>MFKTEFEFPEELKTKLQEHINYFPKKRQAILLCLHEIQNYYGYIPPESLKPLADMLELPLNHVEGVVAFYDMFDREDKAKYRIRVCVSIVCHLMGTNKLLKALENILGIKPGEVTPDGKFKIVPVQCLGACSEAPVFMVNDDEYKFESEVQLNEILSRYT[2x];>MRSYPAIPRIYAETTLNMLLKRAKKPRVHSIDEYLKDGGYQALEKALNMSPEEIIDWVDKSTLRGRGGAGFPTGKKWKFAVQNPGPRYFICNADESEPGTFKDRIIIERDPHLLIEGIIISSYAIGANEAYIYIRGEYPAGYYILRDAIEEAKKKGFLGKNILGSGFDLEIYVARGAGAYICGEETALIESLEGKRGHPRLKPPYPVQKGLWGKPTVVNNVETIANVPFIISMGWEEYRYIGPSDYAGPKLFPVSGKVKKPGVYELPMNTTLREVIFKYAGGTLGNKKVKAVFSGALDCFSSEELDIPMDYSPLGFGGTGTVIVLTEEDDIVEAALKIAEFYEHETCGQCTPCRVGCYEQANLLEKIYKGEATEQDWEGFDFVNRNIQPTSICGLGAVAGRLIRQTLEKFPEEWEKYRKKSASLPLAGHHHHHH[2x]

Complex I couples the transfer of two electrons from NADH to ubiquinone (Q) with the translocation of four protons across the membrane. The L-shaped complex is structured into a peripheral arm that protrudes into the aqueous milieu and catalyzes electron transfer with one FMN and 8–10 iron–sulfur ([Fe–S]) clusters, and a membrane arm embedded in the lipid bilayer that mediates proton translocation. We have determined structures of the electron-input module of complex I from the hyperthermophilic bacterium Aquifex aeolicus, encompassing subunits NuoE and NuoF that contain the FMN cofactor, the [4Fe–4S] cluster N3, and the [2Fe–2S] cluster N1a, respectively, both in the air-oxidized and dithionite-reduced states at resolutions up to 1.8 Å. Here, we show that the redox state of N1a regulates NADH oxidation in complex I by inducing a conformational change close to the NADH-binding site.

To determine the mode of nucleotide binding, crystals of NuoEF were soaked with NAD+, with NADH and with NADH plus dithionite, leading to refined models at 2.0, 1.8, and 1.9 Å resolution, respectively. The structures of NADH and NADH plus dithionite-reduced NuoEF were virtually identical. Noteworthy, in the NAD+-bound state, the peptide bond between E95F and S96F faces the FMN as in the oxidized protein without nucleotide, while in the NADH-bound state, the peptide bond is pointing toward the loop coordinating N1a as it is in the structure of the reduced protein without nucleotide. Remarkably, the reduced nicotinamide group penetrates significantly deeper into the binding pocket than its oxidized form placing it in an optimal position for hydride transfer. The amide carbon atom protrudes 1.65 Å deeper into the binding pocket changing its distance to the Cα carbon atom of Glu95F from 5.37 Å to 4.03 Å. The two positions of the nicotinamide in the binding pocket are here called tight (NADH in reduced NuoEF) and loose (NAD+ in oxidized NuoEF). Water molecules that are here resolved for the first time play an important role in substrate binding by forming hydrogen bonds between NADH and NuoF. The E97F side chain binds the NO2' of NADH by a connecting water molecule. One water molecule bridges the backbone amide of G394F and the side chain of E184F with the NO1 of NADH. In NuoEF, the carbonyl group faces cluster N1a in the reduced state enabling binding of the nicotinamide in the tight position.Here we describe efficient routes starting from validated parallel and antiparallel peptide assemblies to design two families of α-helical barrel proteins with central channels that bind small molecules. Computational designs are seeded by the sequences and structures of defined de novo oligomeric barrel-forming peptides, and adjacent helices are connected by loop building. For targets with antiparallel helices, short loops are sufficient. However, targets with parallel helices require longer connectors; namely, an outer layer of helix–turn–helix–turn–helix motifs that are packed onto the barrels.

Encouraged by the successful design of sc-apCC-6 and sc-CC-7, we extended the seeded design approaches to target α-helical barrel proteins with five, six and eight central helices. By contrast, the six- and eight-helix-based targets bound dye, consistent with accessible cavities, which were confirmed by SEC-SAXS and X-ray crystal structures solved using molecular replacement. Together, these additional designs delivered the de novo proteins sc-CC-5, sc-CC-6 and sc-CC-8. The five-helix-based proteins showed no dye binding, although an X-ray crystal structure revealed an open barrel. Thus, the cavities of five-helix-based barrels appear to be too narrow to accommodate dye. For the parallel targets, the experimental structures show minor fraying at the C termini of the inner helices compared with the seeds and models, which appears to improve the packing of the external three-helix bundles. However, the symmetry of the central parallel helices is maintained. The backbone RMSD values for the repeating helix–turn–helix–turn–helix motifs are ≤0.5 Å, which is expected given the low sequence variation in the loops and the hydrophobic cores of these buttressing helices.

> GSHMEIAATLQEIAKTLAEIAITLAEIAKTLKPESEEAKKAEEEAEKAAKEVEEAIKYAKEHPNSLEAVAKTLQAIAKTLATIAKTLAYIAKTLKPESEEAEKAEEEAKKAAERTEKAIKYAQAHPNSLEAVAKTLLAIAWTLAVIAWTLAYIAKTLDPESEEAEKAKKAAEEAKKKVEEAEKIAQKDPESLEAVAKTLAAIAATLAVIAKTLAYIAKTLDPKSEEAKKAKEKAEAAAKKAAEAIEKAEKDPESLEAIAETLKAIADTLKVIAETLKTIAKTLK> MSSEKEYVEMLDRLYSKLPEKGRKEGTQSLPNMIILNIGNTTIIRNFAEYCDRIRREDKICMKYLLKELAAPGNVDDKGELVI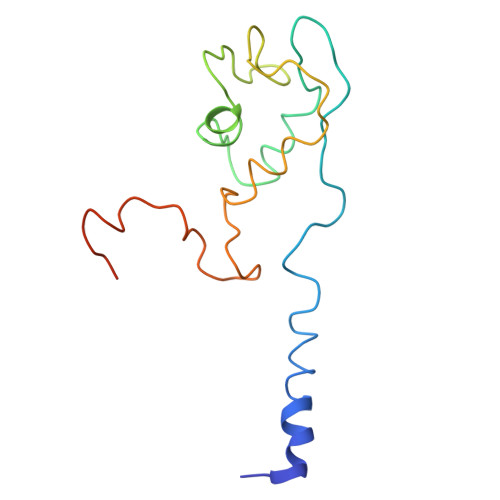QGKFSSQVINTLMERFLKAYVECSTCKSLDTILKKEKKSWYIVCLACGAQTPVKPL>GSHMQFIEGKDYQTVASAQLSTNKDKTPLITEFFSYGCPWCYKIDAPLNDWATRMGKGAHLERVPVVFKPNWDLYAKAYYTAKTLAMS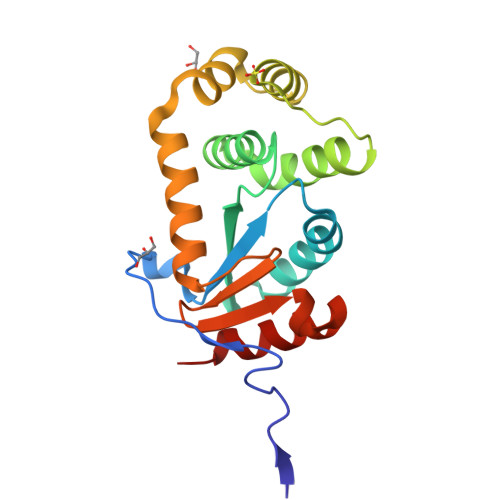DKMNPILFKAIQEDKNPLATKQSMVDFFVAHGVDREIAKSAFENSPTIDMRVNSGMSLMAHYQINAVPAFVVNNKYKTDLQMAGSEERLFEILNYLVRKSA[3x]>[2x]VIPPISCPENEKGPFPKNLVQIKSNKDKEGKVFYSITGQGADTPPVGVFIIERETGWLKVTEPLDRERIATYTLF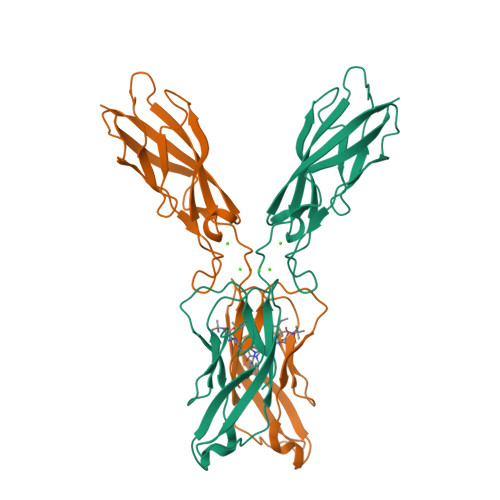SHAVSSNGNAVEDPMEILITVTDQNDNKPEFTQEVFKGSVMEGALPGTSVMEVTATDADDDVNTYNAAIAYTILSQDPELPDKNMFTINRNTGVISVVTTGLDRESFPTYTLVVQAADLQGEGLSTTATAVITVTD> GFD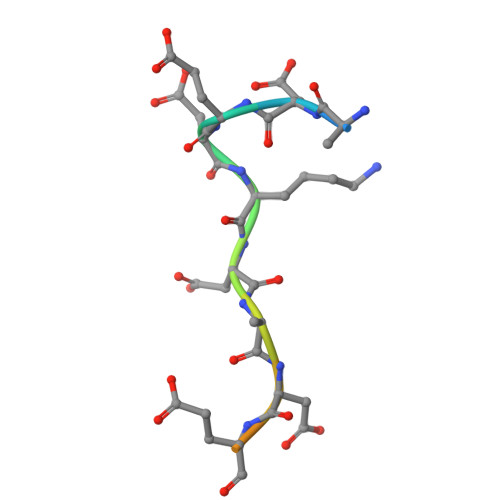EDKDEDEGSPGG> GSRAYSFKVVLLGEGCVGKTSLVLRYCENKFNDKHITTLQASFLTKKLNIGGKRVNLAIWDTAGQERFHALGPIYYRDSNGAILVYDITDEDSFQKVKNWVKELRKMLGNEICLCIVGNKID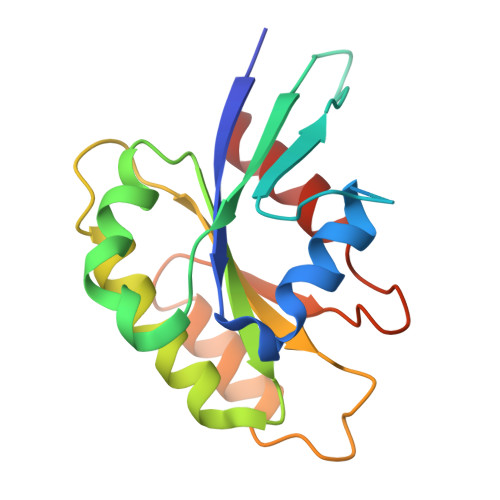LEKERHVSIQEAESYAESVGAKHYHTSAKQNKGIEELFLDLCKRMIET>[4x]GSMEGPAGYLRRADVAQLTQELGTAFFQQQQLPAAMADTFLEHLCLLDIDSEPVAARSTSIIATIGPASRSVERLKEMIKAGMNIARLNFSHGSHEYHAESIANVREAVESFAGSPLSYRPVAIALDTKGPGSGPGLSEQDVRDLRFGVEHGVDIVFASFV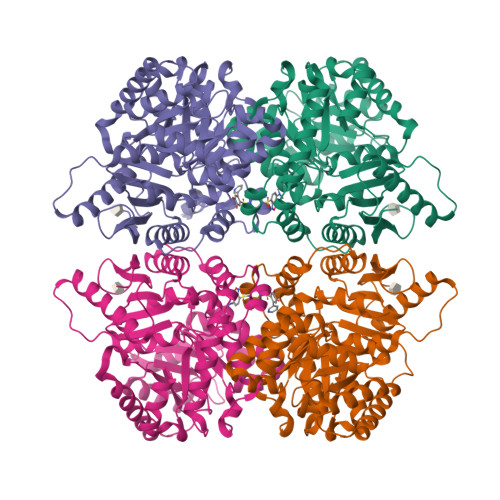RKASDVAAVRAALGPEGHGIKIISKIENHEGVKRFDEILEVSDGIMVARGDLGIEIPAEKVFLAQKMMIGRCNLAGKPVVCATQMLESMITKPRPTRAETSDVANAVLDGADCIMLSGETAKGNFPVEAVKMQHAIAREAEAAVYHRQLFEELRRAAPLSRDPTEVTAIGAVEAAFKCCAAAIIVLTTTGRSAQLLSRYRPRAAVIAVTRSAQAARQVHLCRGVFPLLYREPPEAIWADDVDRRVQFGIESGKLRGFLRVGDLVIVVTGWRPGSGYTNIMRVLSIS Glycoside hydrolase family 7 (GH7) CBHs have been identified as the major protein secreted under cellulase-inducing conditions in several different fungi and play a key role in the degradation of plant biomass, both industrially and in nature. They act processively from the reducing end of a cellulose chain. The most significant structural feature of GH7 CBHs is the presence of a 50 Å long cellulose-binding tunnel in which up to 11 subsites for binding of glucose residues from a cellulose chain have been identified. In this study, we report the crystallization, structural determination and biochemical characterization of H. grisea var. thermoidea Cel7A (HgtCel7A).

The C-terminal linker–CBM1 part was proteolytically removed from the full-length HgtCel7A with papain and the isolated catalytic domain was crystallized, yielding crystals belonging to space group P212121 with two protein molecules, chains A and B, in the asymmetric unit. The two noncrystallographically related protein molecules in the asymmetric unit are practically identical along the β-sandwich core of the structure, but deviate at extended loops that enclose the active site, probably owing to different crystal packing. However, two residues at the C-terminus (438–439) were not visible and are not present in the final model of chain A. One loop that folds back onto the globular domain in chain A to enclose the tunnel at subsites −3/−4 (hereafter called loop B2), appears to be open in chain B and is partly disordered. On the other hand, the last two residues of the catalytic domain, Pro438 and Gly439, show clear density and are included in chain B. The N-terminal glutamine residue is cyclized to pyroglutamate (PCA1) in both chains, and all 18 cysteines form disulfide bonds. N-Glycosylation is evident at Asn271 in chain A, with density for one N-acetylglucosamine residue (NAG), but the density is not clear enough to place an NAG at the corresponding position in chain B. In chain B, the loop is open and partially disordered, with insufficient density to build residues 193–200, probably owing to interference by crystal contacts with a neighbouring protein molecule that prevents closure of the loop. Loop B3 adopts a new conformation where Tyr248 points into subsite +2 of the active site, which has not been observed previously in any GH7 structure. The structure of HgtCel7A indicates that the loops that surround and define the cellulose-binding path through the enzyme have higher flexibility and mobility relative to those of HjeCel7A. The long and remarkably mobile loop B2 is anchored by a salt bridge between Glu191 and Arg206 at the N- and C-termini of the loop.

>QQACSLTTERHPSLSWKKCTAGGQCQTVQASITLDSNWRWTHQVSGSTNCYTGNKWDTSICTDAKSCAQNCCVDGADYTSTYGITTNGDSLSLKFVTKGQHSTNVGSRTYLMDGEDKYQTFELLGNEFTFDVDVSNIGCGLNGALYFVSMDADGGLSRYPGNKAGAKYGTGYCDAQCPRDIKFINGEANIEGWTGSTNDPNAGAGRYGTCCSEMDIWEANNMATAFTPHPCTIIGQSRCEGDSCGGTYSNERYAGVCDPDGCDFNSYRQGNKTFYGKGMTVDTTKKITVVTQFLKDANGDLGEIKRFYVQDGKIIPNSESTIPGVEGNSITQDWCDRQKVAFGDIDDFNRKGGMKQMGKALAGPMVLVMSIWDDHASNMLWLDSTFPVDAAGKPGAERGACPTTSGVPAEVEAEAPNSNVVFSNIRFGPIGSTVAGLPG[2x]> AMMIGIIGAMEE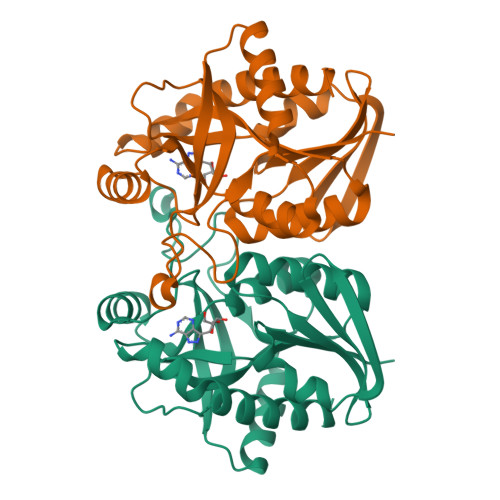EVTILKNKLTQLSEISVAHVKFYTGILKDREVVITQSGIGKVNAAISTTLLINKFKPDVIINTGSAGALDESLNVGDVLISDDVKYHDADATAFGYEYGQIPQMPVAFQSSKPLIEKVSQVVQQQQLTAKVGLIVSGDSFIGSVEQRQKIKKAFPNAMAVEMEATAIAQTCYQFNVPFVVVRAVSDLANGEAEMSFEAFLEKAAVSSSQTVEALVSQL> GGAGGGAAAAGUUAUCAGGCAUGCACCUGGUAGCUAGUCUUUAAACCAAUAGAUUGCAUCGGUUUAAAAGGCAAGACCGUCAAAUUGCGGGAAAGGGGUCAACAGCCGUUCAGUACCAAGUCUCAGGGGAAACUUUGAGAUGGCCUUGCAAAGGGUAUGGUAAUAAGCUGACGGACAUGGUCCUAACCACGCAGCCAAGUCCUAAGUCAACAGAUCUUCUGUUGAUAUGGAUGCAGUUCACAGACUAAAUGUCGGUCGGGGAAGAUGUAUUCUUCUCAUAAGAUAUAGUCGGACCUCUCCUUAAUGGGAGCUAGCGGAUGAAGUGAUGCAACACUGGAGCCGCUGGGAACUAAUUUGUAUGCGAAAGUAUAUUGAUUAGUUUUGGAG

The self-splicing Tetrahymena thermophila group I intron, the first catalytic RNA found, and its multiturnover ribozyme derivative (herein referred to as TET) are well-established model systems used for decades to dissect general principles of RNA folding and catalysis. TET catalyzes the cleavage of a substrate strand using an exogenous guanosine nucleophile. This ~125-kDa ribozyme folds into a compact structure with an internal core of stacked helices stabilized by tertiary contacts between surrounding peripheral domains. Several intermediates have been identified in the folding pathway of TET, including a long-lived misfolded state (referred to as “M”), which can be experimentally accumulated.

In contrast, the second class (blue), which was refined to 3.9 Å, does not fit the structure of N and revealed major differences in the core near the functionally important P7 helix, which contains the conserved guanosine-binding site, indicating that this class likely corresponds to the M state. The final model of M reveals a core topology that diverges from that of N. Whereas in N, the single strand J8/7 is “on top” of J7/3 (which joins helices P7 and P3) as seen from the orientation shown in Fig. 2C, in M J8/7 passes “under” J7/3. Further, the position of J8/7 in M strongly suggests that it docks into the major groove of P3, largely differing from its position away from the major groove of P3 in N; however, the resolution of the structure of M in this area is not sufficiently high to unambiguously describe the specific interactions made between J8/7 and P3. The entanglement of J8/7 is accompanied by a ~90° rotation of P7, likely induced by the new position of J8/7 that constrains proper placement of P7. Consistent with previous observations, long-range tertiary contacts are maintained, although large rearrangements occur within the core. In M, the P1 docking site is partially occupied by P7, which is rotated ~90° and moved by several angstroms relative to N. Thus, the rotated P7 effectively blocks P1 docking, which is an essential step early in the catalytic cycle. Last, as the guanosine-binding site is contained within P7, the large rotation and displacement of this helix would cause the bound guanosine to be in a different position relative to N, even if P1 was able to dock. Visual inspection shows that this topological error cannot be resolved locally and requires major unfolding of the ribozyme (vide infra), consistent with the hours-long time scale at which the M to N transition occurs.> DELYRQSLEIISRYLREQATGAKDTKPM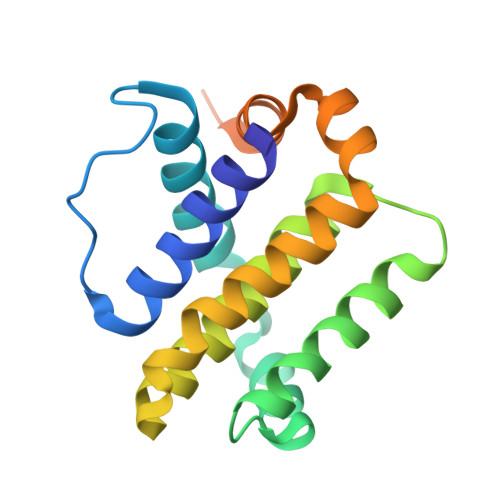GRSGATSRKALETLRRVGDGVQRNHETAFQGMLRKLDIKNEDDVKSLSRVMIHVFSDGVTNWGRIVTLISFGAFVAKHLKTINQESCIEPLAESITDVLVRTKRDWLVKQRGWDGFVEFFHVEDLEGGIRNVLLAFAGVAGVGAGLAYLIR> GPLGSPEFIFDSFLNELHSDITKRGGSPLPLPEGLEECRSSKSSSVIQSWLWDVPGFRRWRVTRLDAGDSLQVFNSVAYPDYNYDHPLMGVDLLWFGARQKLVAVLDFQPLVQDKDYLDRYFSGLKELNQRFPDLNGEETMRSFDPNQYFSSWLLFCRGGAEQADLSLPKAFSAFLKAYWDLHDNAKSIPSTIPPEEVKNLQDKYDIYSA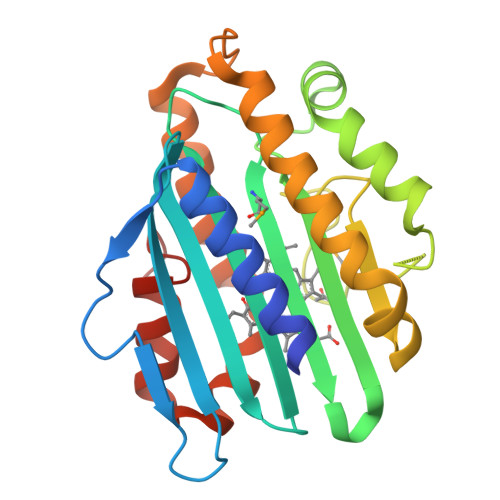ERDPAHGLFTSHFGKDWSNRFLHEFLFPASSSHK> MKKAVINGEQIRSISDLHQTLKKELALPEYY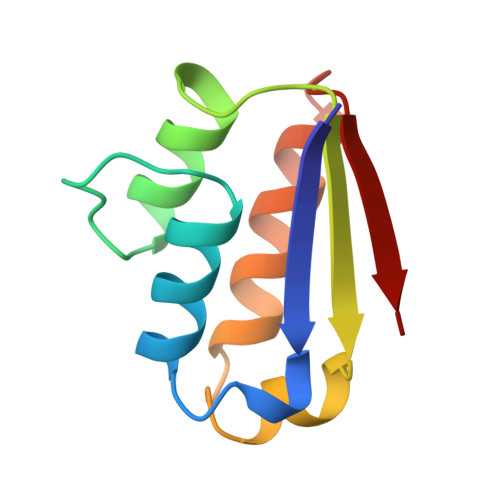GENLDALWDCLAGWVEYPLVLEWRQFEQSKQLTENGAESVLQVFREAKAEGCDITIILS> NL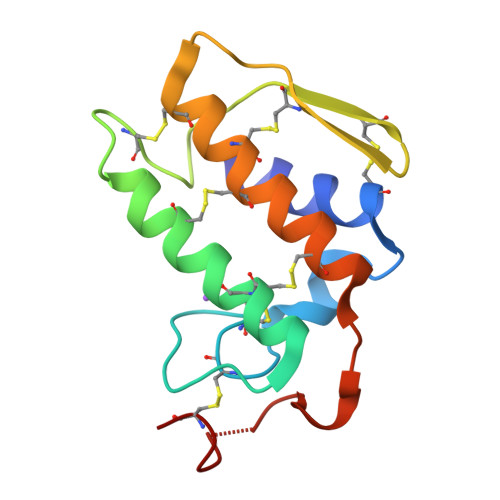IQFKNMIQCAGTRIWTAYVAYGCYCGKGGSGTPVDELDRCCYTHDHCYNEAEKIPGCNPNIKTYSYTCTQPNLTCTDSADTCAQFLCECDRTAAICFASAPYNSNNIMLSSSTSCQ>MDLPPDSRTALRDWLTEQLADLLGEPLADVRALADDDDLLGCGLDSIRLMYLQERLRARGSTLDFAQLAQRPCLGAWLDLLACADRLSAPATVALPTAQDRDQPFELSSVQQAYWLGRGAGEVLGNVSCHAFLEFRTRDVDPQRLAAAAECVRQRHPMLRARFLDGRQQILPTPPLSCFDLQDWRTLQVDEAERDWQALRDWRAHECLAVERGQVFLLGLVRMPGGEDRLWLSLDLLAADVESLRLLLAELGVAYLAPERLAEPPALHFADYLAHRAAQRAEAAARARDYWLERLPRLPDAPALPLACAPESIRQPRTRRLAFQLSAGESRRLERLAAQHGVTLSSVFGCAFALVLARWSESAEFLLNVPLFDRHADDPRIGEVIADFTTLLLLECRMQAGVSFAEAVKSFQRNLHGAIDHAAFPALEVLREARRQGQPRSAPVVFASNLGEEGFVPAAFRDAFGDLHDMLSQTPQVWLDHQLYRVGDGILLAWDSVVGLFPEGLPETMFEAYVGLLQRLCDSAWGQPADLPLPWAQQARRALLNGQPACATARTLHRDFFLRAAEAPDADALLYRDQRVTRGELAERALRIAGGLREAGVRPGDAVEVSLPRGPQQVAAVFGVLAAGACYVPLDIDQPPARRRLIEEAAGVCLAITEEDDPQALPPRLDVQRLLRGPALAAPVPLAPQASAYVIYTSGSTGVPKGVEVSHAAAINTIDALLDLLRVNASDRLLAVSALDFDLSVFDLFGGLGAGASLVLPAQEQARDAAAWAEAIQRHAVSLWNSAPALLEMALSLPASQADYRSLRAVLLSGDWVALDLPGRLRPRCAEGCRLHVLGGATEAGIWSNLQSVDTVPPHWRSIPYGRPLPGQAYRVVDTHGRDVPDLVVGELWIGGASLARGYRNDPELSARRFVHDAQGRWYRTGDRGRYWGDGTLEFLGRVDQQVKVRGQRIELGEVEAALCAQAGVESACAAVLGGGVASLGAVLVPRLAPRAEGSMDLPAAQPFAGLAEAEAVLTREILGALLEAPLELDDGLRRRWLDWLADSAASALPSLDEALRRLGWQAAGLTA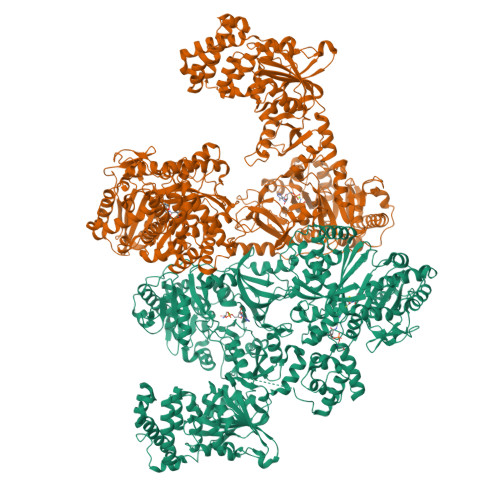MGNALRGLLAGEQAPAALLLDPWLAPQAVAARLPDGREALARLLEALPTPAAGERLRVAVLDTRAGLWLDQGMASLLRPGLELTLFERSRVLLDAAATRLPERIVVQALDDGLLPAEHLGRYDRVISFAALHAYEASREGLALAAALLRPQGRLLLVDLLCESPLALLGAALLDDRPLRLAELPSLLADLAAAGLAPRCLWRSERIALVEALAPGLGLDAAALQAGLEQRLPQAMRPERLWCLPSLPLNGNGKVDRRRLAESMTRALGECRHEPSAEEPLEAHEQALAECWEAVLKRPVRRREASFFSLGGDSLLATRLLAGIRERFGVRLGMADFYRQPTLAGLARHLQVQTVEIEETQLEEGVLHHHHHHLPSWSHPQFEK[2x]> AAAAA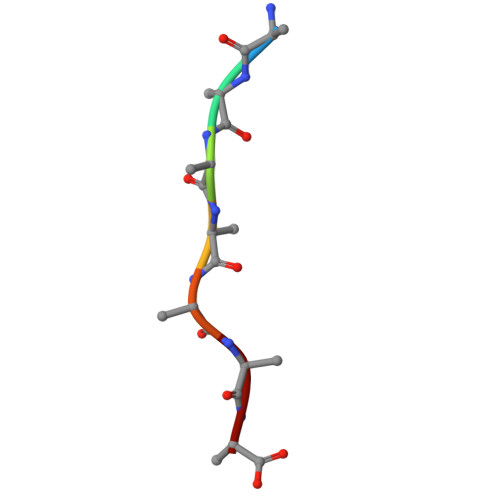AA> CTSIVAQDSRGHIYHGRNLDYPFGNVLRKLTVDVQFLKNGQIAFTGTTFIGYVGLWTGQSPHKFTVSGDERDKGWWWENAIAALFRRHIPVSWLIRATL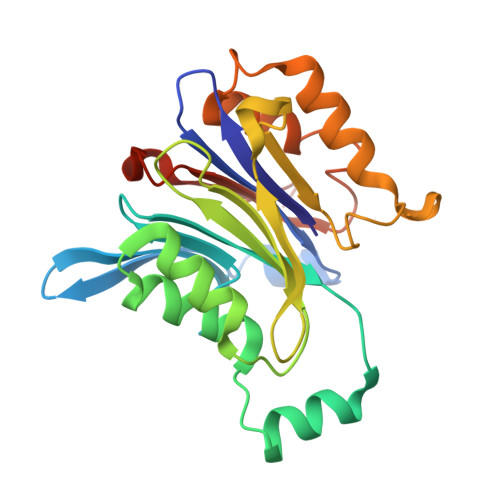SESENFEAAVGKLAKTPLIADVYYIVGGTSPREGVVITRNRDGPADIWPLDPLNGAWFRVETNYDHWKPAPKEDDRRTSAIKALNATGQANLSLEALFQILSVVPVYNNFTIYTTVMSAGSPDKYMTRIRNPSRK> HHHHHHDWVIPPIKVSENERGPFPKRLVQIKSNKDRFNKVYYSITGQGADNPPQGVFRIEWETGWMLVTRPLDREEYDKYVLSSHAVSENGSPVEEPMEITINVIDQNDNRPKFTQDVFRGSVREGVQPGTQVMAVSATDEDDNIDSLNGVLSYSILKQDPEEPIPNLFTINRETGVISLIGTGLDREKFPEYTLTVQATDLEGAGLSVEGKAIIQITDANDNAPIFDPKTYTALVPENEIGFEVQRLSVTDLDMPGTPAWQAVYKIRVNEGGFFNITTDPESNQGILTTAKGLDFELRKQYVLQITVENAEPFSVPLPTSTATVTVTVEDVNEAPFFVPAVSRVDVSEDLSRGEKIISLVAQDPDKQQIQKLSYFIGNDPARWLTVNKDNGIVTGNGNLDRESEYVKNNTYTVIMLVTD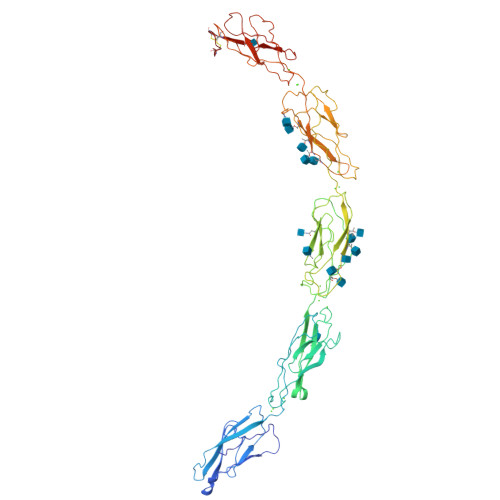DGVSVGTGTGTLILHVLDVNDNGPVPSPRVFTMCDQNPEPQVLTISDADIPPNTYPYKVSLSHGSDLTWKAELDSKGTSMLLSPTQQLKKGDYSIYVLLSDAQNNPQLTVVNATVCSCEGKAIKCQ The Lon protease is a AAA+ protein found in prokaryotes, archaea, and eukaryotic organelles. Lon is involved in cellular protein homeostasis by degrading damaged or misfolded abnormal proteins, which prevents these unwanted protein species from forming toxic aggregates. Lon is known to form a homohexamer; each protomer is composed of multiple domains, including an N-terminal substrate-binding globular domain (NGD), a long-helix domain (LH), a three-helix bundle (3H), a AAA+ ATPase module, and a protease domain. We show here, using cryo-electron microscopy (cryo-EM), that the activation process of the Lon AAA+ protease may involve a pentameric assembly and a substrate-dependent incorporation of the sixth protomer to form the substrate-pore-loop contacts seen in the translocating state.

To test this hypothesis, we performed single-particle cryo-EM reconstruction of the proteolytically deficient mutant MtaLon-S678A incubated with ADP and the model substrate α-casein. The pentameric assembly forms a left-handed open-spiral structure. The open-spiral pentamer forms a large gap between the protomers Ob1 and Ob5. The pentamer forms a tensegrity helix triangle (THT), consisting of three overlapping LHs from Ob1, Ob3, and Ob5, forming an interlocked, letter A-shaped structure that tethers together five protomers. In the pentameric assembly, only the pore-loop residues, Tyr397 and Trp431, of the protomers Ob1, Ac4, and Ob5 are accessible to the entry gate lined by Tyr224 and Met217 residues. Notably, they are scattered along a right-handed spiral trajectory.

>[5x]MRLELPVIPLRNTVILPHTTTPVDVGRAKSKRAVEEAMGADRLIFLVAQRDPEVDDPAPDDLYTWGVQAVVKQAMRLPDGTLQVMVEARARAQVTDYIPGPYLRARGEVFSEIFPIDEAVVRVLVEELKEAFEKYVANHKSLRLDRYQLEAVKGTSDPAMLADTIAYHATWTVAEKQEILELTDLEARLKKVLGLLSRDLERFELDKRVAQRVKEQMDTNQREYYLREQMKAIQKELGGEDGLSDLEALRKKIEEVGMPEAVKTKALKELDRLERMQQGSPEATVARTYLDWLTEVPWSKADPEVLDINHTRQVLDEDHYGLKDVKERILEYLAVRQLTQGLDVRNKAPILVLVGPPGVGKTSLGRSIARSMNRKFHRISLGGVRDEAEIRGHRRTYIGAMPGKLIHAMKQVGVINPVILLDEIDKMSSDWRGDPASAMLEVLDPEQNNTFTDHYLDVPYDLSKVFFITTANTLQTIPRPLLDRMEVIEIPGYTNMEKQAIARQYLWPKQVRESGMEGRIEVTDAAILRVISEYTREAGVRGLERELGKIARKGAKFWLEGAWEGLRTIDASDIPTYLGIPRYRPDKAETEPQVGTAQGLAWTPVGGTLLTIEVAAVPGSGKLSLTGQLGEVMKESAQAALTYLRAHTQDYGLPEDFYNKVDLHVHVPDGATPKDGPAAGITMATAIASALSRRPARMDIAMTGEVSLRGKVMPIGGVKEKLLAAHQAGIHKIVLPKDNEAQLEELPKEVLEGLEIKLVEDVGEVLEYLLLPEPTMPPVVQPSDNRQQPGAGA>MEAGITGTWYNQLGSTFIVTAGADGALTGTYVTARGNAESRYVLTGRYDSAPATDGSGTALGWTVAWKNNYRNAHSATTWSGQYVGGAEARINTQWLLTSGTTEENAGYSTLVGH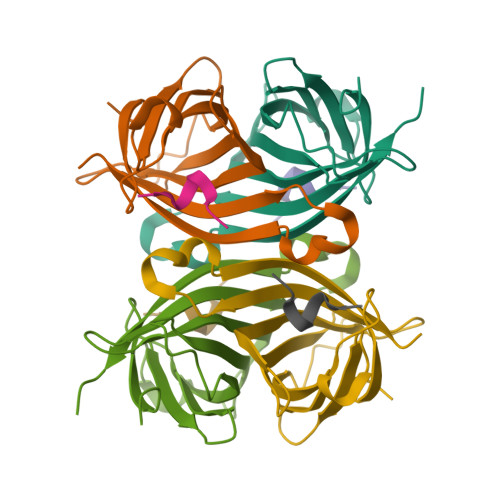DTFTKVKPSAAS[2x];>XSAWSHPQFEKX[2x]3-CHLOROPROPANOL | C3 H7 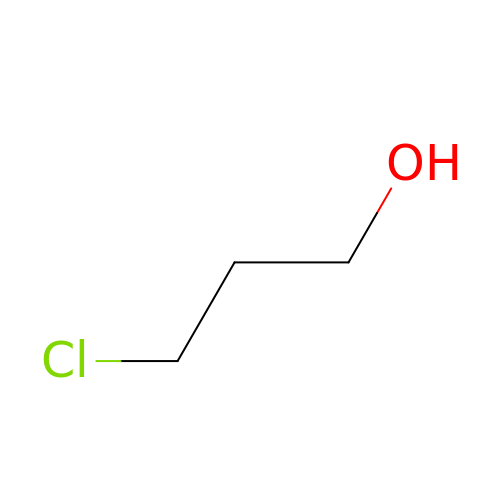Cl O | LAMUXTNQCICZQX-UHFFFAOYSA-N>MTINYHELETSHGRIAVRESEGEGAPLLMIHGNSSSGAIFAPQLEGEIGKKWRVIAPDLPGHGKSTDAIDPDRSYSMEGYADAMTEVMQQLGIADAVVFGWSLGGHIGIEMIARYPEMRGLMITGTPPVAREEVGQGFKSGPDMALAGQEIFSERDVESYARSTC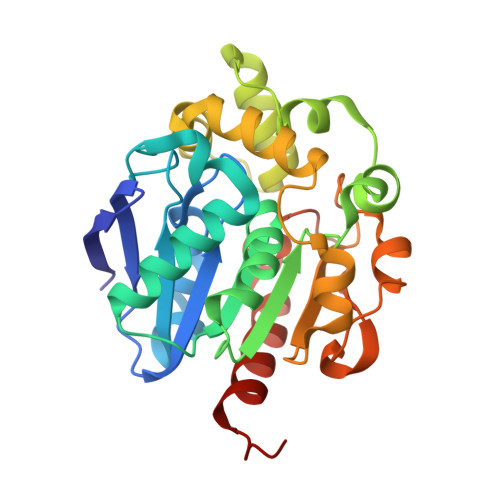GEPFEASLLDIVARTDGRARRIMFEKFGSGTGGNQRDIVAEAQLPIAVVNGRDGPFVELDFVSKVKFGNLWEGKTHVIDNAGHAPFREAPAEFDAYLARFIRDCTQLEHHHHHH[2x]> GSHAIVKVTDADFDSKVESGVQLVDFWATWCGSCKMIAPVLEELAADYEGKADILKLDVDENP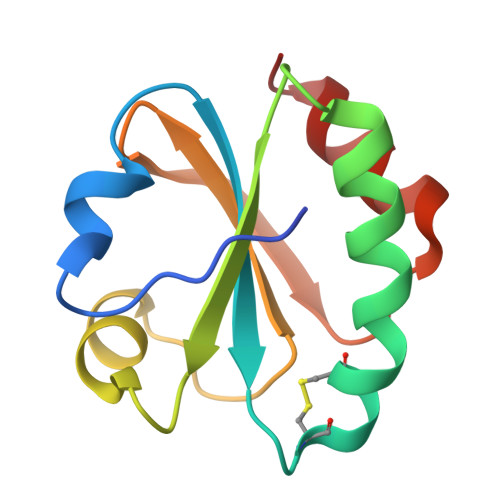STAAKYEVMSIPTLIVFKDGQPVDKVVGFQPKENLAEVLDKHL> MSLPLRHALENVTSVDRILEDLLVRFIIN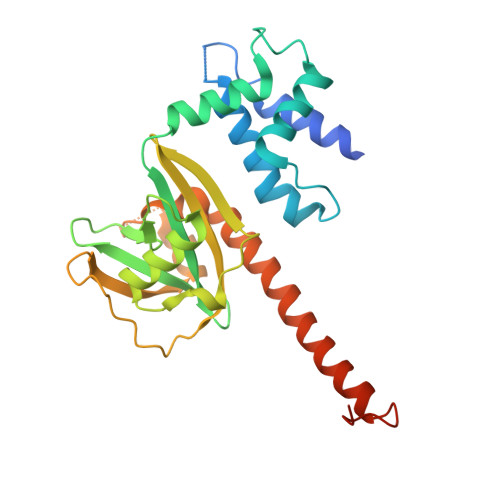CPNEDLSSVERELFHFEEASWFYTDFIKLMNPTLPSLKIKSFAQLIIKLCPLVWKWDIRVDEALQQFSKYKKSIPVRGAAIFNENLSKILLVQGTESDSWSFPRGKISKDENDIDCCIREVKEEIGFDLTDYIDDNQFIERNIQGKNYKIFLISGVSEVFNFKPQVRNEIDKIEWFDFKKISKTMYKSNIKYYLINSMMRPLSMWLRHQRQIKNEDQLKSYAEEQLKLLLGITKEEQIDPGRHHHHHH> SCSMPLGMQNKAISDSQITASSHLSNIFATWSPSQARLHLQGRTNAWRPRVSSAEEWLQVDLQKTVKVTGITTQGVKSLLSSMYVKEFLVSSSQDGRRWTLFLQDGHTKVFQGNQDSSTPVVNALDPPLFTRYLRIHPTSWAQHIALRLEVLGCEAA

Factor VIII (fVIII) is an essential cofactor in the intrinsic pathway of the blood coagulation cascade in which activated fVIII (fVIIIa) associates to phosphatidyl-L-serine (PS) presented on the surface of activated platelet membranes. At the PS membrane surface, fVIIIa binds to activated factor IX (fIXa), forming the active intrinsic “tenase” complex which catalyzes factor X activation. Association of fVIIIa to membranes is coordinated by two tandem carboxy-terminal C domains. The C domains of fVIII, termed C1 and C2, are 16 kDa β-sandwich folds that share 66% sequence identity.

Lastly, we determined the X-ray crystal structure of the porcine fVIII C2 domain bound to o-phospho-L-serine, the polar headgroup of PS, which binds to a basic cleft and makes charge-charge contact with R2320. The structure of C2:OPLS complex was determined to 1.3 Å resolution and refined to an Rwork and Rfree of 13.5% and 15.7%, respectively. Analysis of surface electrostatics illustrates how OPLS binds to a positively charged pocket in the C2 domain centered on residue R2320. Real space modeling of the OPLS ligand positions the carboxy end of OPLS 3.2 Å and 3.0 Å from the R2320 guanidino group. The carbon backbone of OPLS extends away from the core of the C2 domain, adjacent to the solvent exposed hydrophobic loops previously demonstrated to be an important determinant for PS membrane binding. Within the structure, a 3.3 Å hydrogen bond is observed between the S2289 hydroxyl group and the amino moiety of OPLS while N2217 forms two amide nitrogen contacts to the phosphate group at 3.1 and 3.4 Å. A single interaction exists between the Q2213 amide-nitrogen and both carboxyl oxygens of OPLS with additional polar interactions between amide side chains of Q2213 and N2217 at 3.7 Å. The OPLS group is situated between two loops, L2210-G2214 and S2250-S2253, forming noncovalent interactions with Q2213, N2217, S2289, and R2320. Although the structure is high resolution, poor electron density is observed for the two β-hairpin loops, indicating high dynamic character. Two alternative conformations for the 2197–2200 loop were resolved in the final model to account for the flexible nature of these hydrophobic loops.Herein, we design metalloglycosidases by constructing a hydrolytically active Zn-binding site within a barrel-shaped outer membrane protein OmpF. We supposed that a protein containing a void space, such as β-barrel outer membrane protein F (OmpF), would be suitable for our study; its overall shape resembles the structure of host compounds, such as cyclodextrin, which may provide a structural basis for various functions, including catalysis, by encompassing guest molecules and forming noncovalent interactions. We inspected the constriction zone of OmpF, the narrowest region, approximately halfway inside the barrel-shaped protein. A coordinatively unsaturated mononuclear Zn-binding site, a common catalytic motif in metallohydrolases, was created by placing three metal-coordinating histidines.

As a result, two triple mutants, R82H/Y102H/R132H (OmpF1) and L83H/Y102H/R132H (OmpF2), were designed as the parent templates. After protein extraction, purification, and refolding, they were isolated as β-barrel trimers, retaining the native overall architecture of OmpF. More importantly, both proteins possess a mononuclear Zn-binding site in the constriction zone. The fourth coordination site was possibly ligated by a water molecule, which is again suitable for our studies. Of note, the empty coordination site of OmpF2 pointed toward the periplasmic side, whereas that of OmpF1 is placed toward the extracellular region. In particular, D113 shows proper orientation and interatomic distance between the terminal oxygen atom and Zn-bound exchangeable ligands as 7.9–9.5 Å and 4.7–5.1 Å in OmpF1 and OmpF2, respectively. In addition, D113E mutation (denoted as /E) altered the glycosidase activities of OmpF variants; OmpF1/E and OmpF2/E showed substantially elevated activities, whereas that of OmpF1Y/E was somewhat reduced. For retaining β-glycosidases, such as OmpF2/E-R2, an acidic residue, possibly D113E, may initiate glycosylation as a nucleophile when Zn-OH2 species acts as a Lewis acid.

>AEIYNKDGNKVDLYGKAVGLHYFSKGNGENSYGGNGDMTYARLGFKGETQINSDLTGYGQWEYNFQGNNSEGADAQTGNKTRHAFAGLKYADVGSFDYGRNHGVVYDALGYTDMLPEFGGDTAYSDDFFVGHVGGVATYRNSNFFGLVDGLNFAVQYLGKNERDTARRSNGDGVGGSISYEYEGFGIVGAYGAADRTNLQEAQPLGNGKKAEQWATGLKYDANNIYLAANYGETRNATPITNKFTNTSGFANKTQDVLLVAQYQFDFGLRPSIAYTKSKAKDVEGIGDVDLVNYFEVGATYYFNKNMSTYVDYIINQIDSDNKLGVGSDDTVAVGIVYQF[3x]trans-cyclohexane-1,4-dicarboxylic acid | C8 H12 O4 | 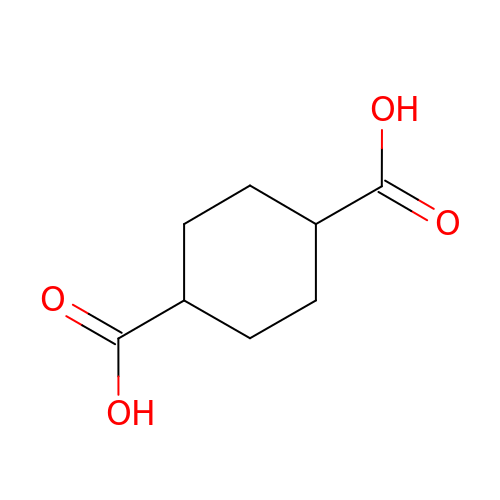PXGZQGDTEZPERC-IZLXSQMJSA-N> DWVIPPINLPENSRGPFPQELVRIRSDRDKNLSLRYSVTGPGADQPPTGIFIINPISGQLSVTKPLDRELIARFHLRAHAVDINGNQVENPIDIVINVIDMNDNRPEFLHQVWNGSVPEGSKPGTYVMTVTAIDADDPNALNGMLRYRILSQAPSTPSPNMFTINNETGDIITVAAGLDREKVQQYTLIIQATDMEGNPTYGLSNTATAVITVTDVNDNPPEFTAMTFYGEVPENRVDVIVANLTVTDKDQPHTPAWNAAYRISGGDPTGRFAILTDPNSNDGLVTVVKPIDFETNRMFVLT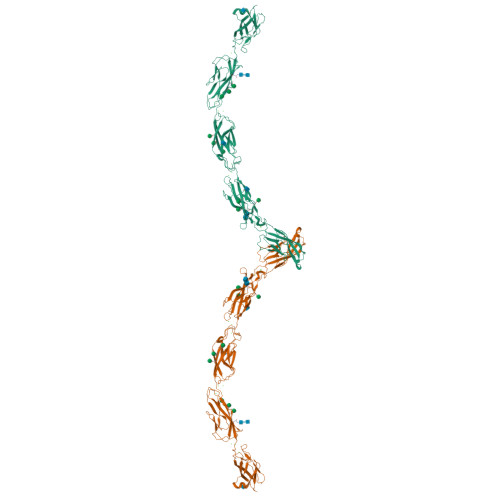VAAENQVPLAKGIQHPPQSTATVSVTVIDVNENPYFAPNPKIIRQEEGLHAGTMLTTLTAQDPDRYMQQNIRYTKLSDPANWLKIDPVNGQITTIAVLDRESPNVKNNIYNATFLASDNGIPPMSGTGTLQIYLLDINDNAPQVLPQEAETCETPEPNSINITALDYDIDPNAGPFAFDLPLSPVTIKRNWTINRLNGDFAQLNLKIKFLEAGIYEVPIIITDSGNPPKSNISILRVKVCQCDSNGDCTDVHHHHHH> ADLTASTTATATLVEPARITLTYKEGAPITIMDNGNIDTELLVGTLTLGGYKTGTTSTSVNFTDAAGDPMYLTFTSQDGNNHQFTTKVIGK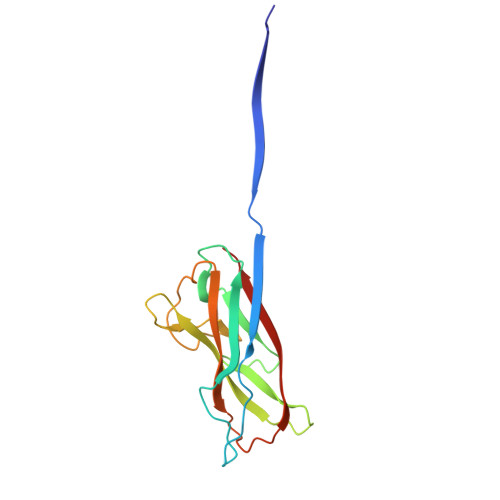DSRDFDISPKVNGENLVGDDVVLATGSQDFFVRSIGSKGGKLAAGKYTDAVTVTVSNQ3-[4-(6-cyclopropylpyridin-3-yl)phenyl]-N-(4-fluorophenyl)oxetane-3-carboxamide 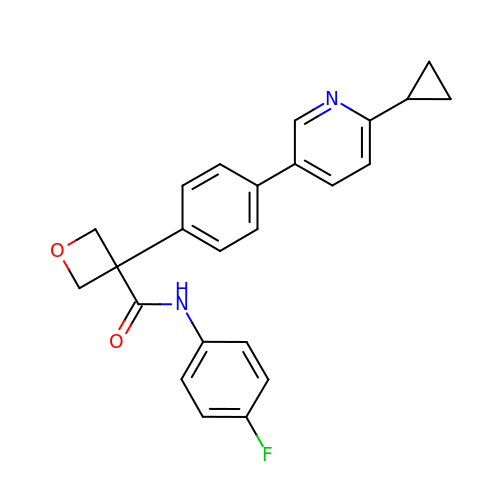| C24 H21 F N2 O2 | DJWKVSDUOMVCDV-UHFFFAOYSA-N>[2x]GDTKEQRILRYVQQNAKPGDPQSVLEAIDTYCTQKEWAMNVGDAKGQIMDAVIREY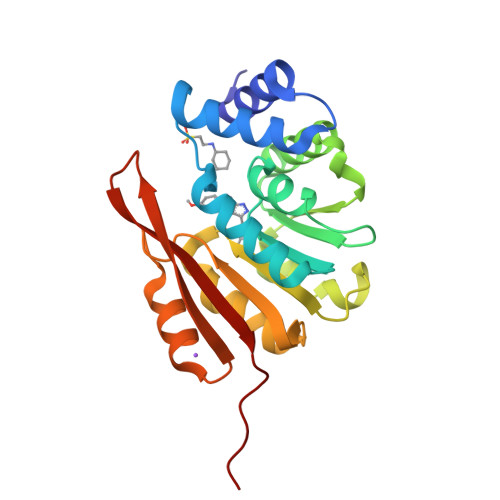SPSLVLELGAYCGYSAVRMARLLQPGARLLTMEINPDCAAITQQMLNFAGLQDKVTILNGASQDLIPQLKKKYDVDTLDMVFLDHWKDRYLPDTLLLEECGLLRKGTVLLADNVIVPGTPDFLAYVRGSSSFECTHYSSYLEYMKVVDGLEKAIYQGPSSPDK> MGPSENDPNLFVALYDFVASGDNTLSIT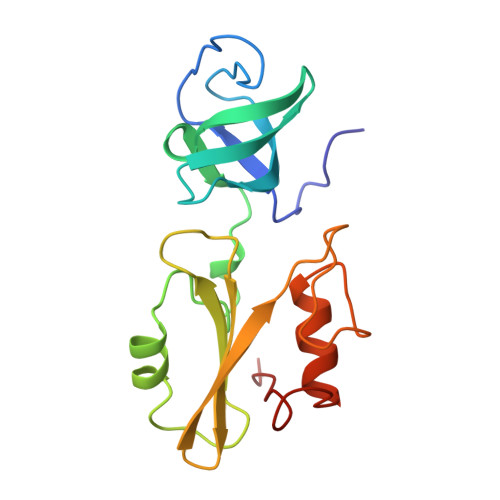KGEKLRVLGYNHNGEWCEAQTKNGQGWVPSNYITPVNSLEKHSWYHGPVSRNAAEYLLSSGINGSFLVRESESSPGQRSISLRYEGRVYHYRINTASDGKLYVSSESRFNTLAELVHHHSTVADGLITTLHYPAP Influenza A virus has two surface glycoproteins, hemagglutinin (HA) and neuraminidase (NA), that act as the major antigens. NA is a type II transmembrane protein that forms a homotetramer. The natural function of NA is to cleave the sialic acids from cellular receptors to facilitate virus release and from newly synthesized HA to prevent virion aggregation. Neuraminidase (NA) of human influenza H3N2 virus has evolved rapidly and been accumulating mutations for more than half-century.

To further examine the structural mechanism of epistasis between K385N and N387K, we determined the crystal structure of NAs from Bil69, SD93, and Mos99 to 1.54 Å, 1.65 Å, and 1.40 Å, respectively. Of note, the structure of SD93 NA was determined in complex with zanamivir. The backbone conformation of the loop that contains residues 385 to 389 is highly conserved between NAs from Bil69, SD93, and Mos99. Although N387K decreased the fitness of Mos99, it reduced the titer of SD93 to below the detection limit. Briefly, we constructed a mutant library for SD93 that contained all possible combinations of 10 mutations (n = 210 = 1024 variants), namely E248G, R249K, I265T, Y336H, R338L, N339D, K344E, S346G, E369K, and G381E, in the genetic background of N387K. Mutations E248G, R249K, Y336N, K344E, and E369K were enriched among variants with a frequency of >0.1% in the post-passaged mutant libraries of both biological replicates, suggesting that they could restore the fitness of N387K in SD93. The pentamutant E248G/R249K/Y336N/K344E/E369K was indeed able to partially restore the virus titer of N387K. The virus titer of E248G/R249K/Y336N/K344E/E369K/N387K could be further increased by the addition of K385N. Our results showed that N387K reduced the Tm of Mos99 NA and SD93 NA by around 5 °C. An interesting observation in this study is that while SD93 NA K385N/N387K mutant has a WT-like thermostability, which indicates proper folding of the protomer, its enzymatic activity is minimal.

> MNPNQKIITIGSVTLTIATICFLMQIAILVTTVTLHFKQYECNSPPNNQVMLCEPTIIERNITEIVYLTNTTIEKEICPKLAEYRNWSKPQCKITGFAPFSKDNSIRLSAGGDIWVTREPYVSCDPGKCYQFALGQGTTLNNRHSNDTVHDRTPYRTLLMNELGVPFHLGTKQVCIAWSSSSCHDGKAWLHVCVTGHDENATASFIYDGRLVDSIGSWSKNILRTQESECVCINGTCTVVMTDGSASERADTKILFIEEGKIVHISPLSGSAQHVEECSCYPRYPGVRCVCRDNWKGSNRPIVDINVKDYSIVSSYVCSGLVGDTPRKNDSSSSSYCRNPNNEKGSHGVKGWAFDDGNDVWMGRTISEELRSGYETFKVIGGWSKPNSKLQINRQVIVDRGNRSGYSGIFSVEGKSCINRCFYVELIRGRKQETEVWWTSNSIVVFCGTSGTYGTGSWPDGGDINLMPI>[4x]AFDYDGPLMKTEVPGPRSRELMKQLNIIQNAEAVHFFCNYEESRGNYLVDVDGNRMLDLYSQISSIPIGYSHPALVKLVQQPQNVSTFINRPALGILPPENFVEKLRESLLSVAPKGMSQLITMACGSCSNENAFKTIFMWYRSKERGESAFSKEELETCMINQAPGCPDYSILSFMGAFHGRTMGCLATTHS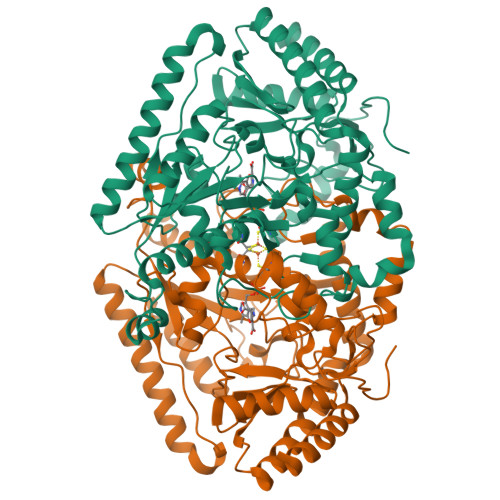KAIHKIDIPSFDWPIAPFPRLKYPLEEFVKENQQEEARCLEEVEDLIVKYRKKKKTVAGIIVEPIQSEGGDNHASDDFFRKLRDISRKHGCAFLVDEVQTGGGSTGKFWAHEHWGLDDPADVMTFSKKMMTGGFFHKEEFRPNAPYRIFNTWLGDPSKNLLLAEVINIIKREDLLSNAAHAGKVLLTGLLDLQARYPQFISRVRGRGTFCSFDTPDESIRNKLISIARNKGVMLGGCGDKSIRFRPTLVFRDHHAHLFLNIFSDILADFK>MVPDNSIPICSDVTKLNFQALIDAQMRHAGKMFDVIMMDPPWQLSSSQPSRGVAIAYDSLSDEKIQNMPIQSLQQDGFIFVWAINAKYRVTIKMIENWGYKLVDEITWVKKTVNGKIAKGHGFYLQH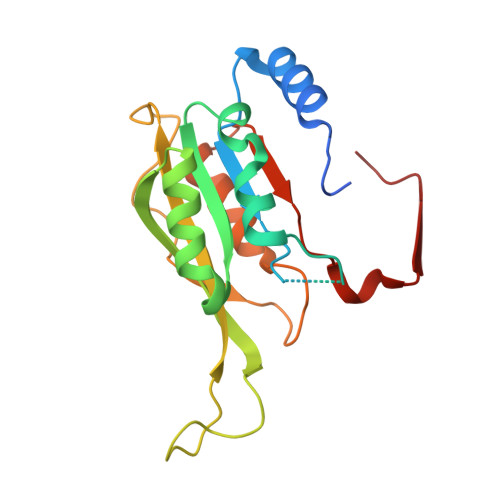AKESCLIGVKGDVDNGRFKKNIASDVIFSERRGQSQKPEEIYQYINQLCPNGNYLEIFARRNNLHDNWVSIGNEL[4x]>MKTLLKNSLTFLLMLMPVLAFAQQAPQIMNVSARQTTSLDGQWKTIVDPFENGYYDYRLKPYDGGYAQDKTYSDKTKLQEYDFETDKLLFVPGDWNTQRPQLYYYEGTVWYRKHFEYSLQPGKRLFLNFGAVNYEAIVWLNGKRLGRHIGGFTPFNFEITNLLKEGTNSLVVKVDNKRLPEAVPTVNADWWNFGGITRPVTLIEMPATYIRDYYVQLAKDDKNMIEGWVQLEGSDKEQKITLDIPELKVKKEVTTDANGYASFLIKSKPILWTPENPKLYAVNLASETDKVSDEIGFRTIRTEG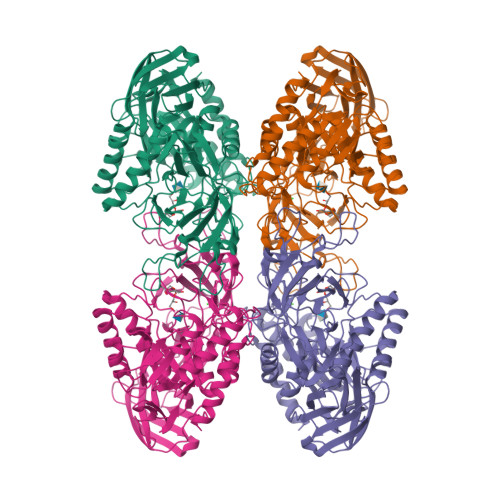IKILLNDKEIFCRGISIHEETPYYSGRAYSKDHAHTLLSWAKELGCNFVRLAHYPHNEEMVREAERMGFLVWSEIPVYWTIHWENKDTYQNAEQQLCDMIARDKNRCNIIIWSIANETPHSKTRLTFLSNLANKARSLDSVRLIGAAMEKEEVQPGVLTVNDPLGELLDIISFNEYVGWYDGDSEKCDRVNWTFDTQKPVFISELGGGALYGHHGSPKERFTEEYQEDLYIRHVNMLKRIPGLAGTTPWILKDFRSPRRHVPEIQDDFNRKGLVSDKGQKKKAFFVLQKWYKELTEAYK[4x]SpoIIE from B. subtilis is an 827-residue protein thought to consist of three domains. It has 10 putative membrane-spanning segments at its N-terminus and a PP2C-type phosphatase domain at its C-terminus. SpoIIE belongs to the metal-dependent protein phosphatase (PPM) family exemplified by human PP2C. The pathway of σF activation begins with the dephosphorylation of SpoIIAA∼ P by SpoIIE and culminates in the displacement of σF from the complex with SpoIIAB by SpoIIAA.

To gain structural insight into Mn2+ chelation in SpoIIE, we sought and obtained crystals of SpoIIE(590–827) from drops prepared from solutions in which the citrate was replaced by acetate and in which the protein was pre-incubated for 30 min with 2 mM MnCl2. The “citrate” and “acetate” crystals are essentially isomorphous, and a domain-swapped dimer is again observed. In the latter structure, we observed a single high-occupancy manganese (Mn2+) ion in the active site. The manganese ion in each active site of SpoIIE is coordinated by the side-chain carboxylates of Asp628, Asp746 and Asp795 with the Asp628 ligand provided by the partner subunit in the domain-swapped dimer. The octahedral coordination and the coordinating ligands (contributed by three carboxylates and two water molecules) are conserved in SpoIIE. The three metal ions in PstP, MspP, STP and tPphA are almost exactly superposed following an overlap of the structures based on protein Cα positions. In this comparison, the single metal ion in the SpoIIE structure superimposes closely with the first of the manganese ions, Mn1, of the bacterial phosphatases as shown for MtPstP in Fig. 5c. There would appear to be capacity in SpoIIE to coordinate a second Mn species, equivalent to Mn2 in the other bacterial phosphatases, since the corresponding protein ligands Asp628, Gly629 and Asp610 are conserved and appropriately situated. There does not however appear to be capacity to bind a third Mn2+, equivalent to Mn3, since only one of the coordinating protein ligands is conserved, this being Asp746 whose equivalent bridges the Mn1 and Mn3 metal ions in the other bacterial phosphatase structures.

>GPAMSYRVSTGAAHAAKGGGLVSGDSYSMMELGARKYAAAISDGMGNGARAHFESNETIKLLEKILESGIDEKIAIKTINSILSLRTTDEIYSTLDLSIIDLQDASCKFLKVGSTPSFIKRGDQVMKVQASNLPIGIINEFDVEVVSEQLKAGDLLIMMSDGIFEGPKHVENHDLWMKRKMKGLKTNDPQEIADLLMEEVIRTRSGQIEDDMTVVVVRIDHNTPKWASIPVPAIFQNKQEIS[2x]>[2x]GHMTHSAY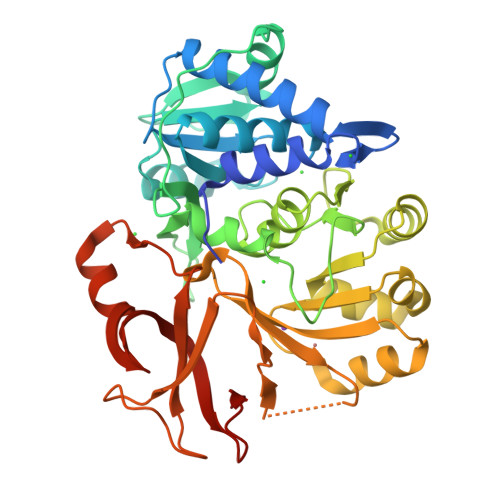VYQLKAVPDIFDEISQRFPDRVALIFDQRKITYRELAEQCSALAAVLQNNCLIKGDIVAIKIERSPELYIFMLALMKIGAVMVPVNSNSPERYIGEVLSAAGARYLISDDVTSVPGGAWHVLSSRTLIQNCTQQRSGNYPVLSADDPALILMTSGSTGKPKSVLIAHRGIARLGLPVPALGNSERDCYLQIADISFAASANEIWMALLTGACLTIAPPGLPDLMALARQIESDNVTMLFLSGGLFRLFVEVSVETLHIPDCVVVSGDFVNPRLFSVAVQAGKAKIFNGLGCTENSAISSLYHIQSAAALSSESPVPVGTPLPLVEMVVFNERLQPCTCGEYGELFIAGAGVALGYSDPQLTAERFITIPYQGTDMLFYRTDDRATYDQDRNIVLVGRG> MWIVFDVDGVLIDVRESYD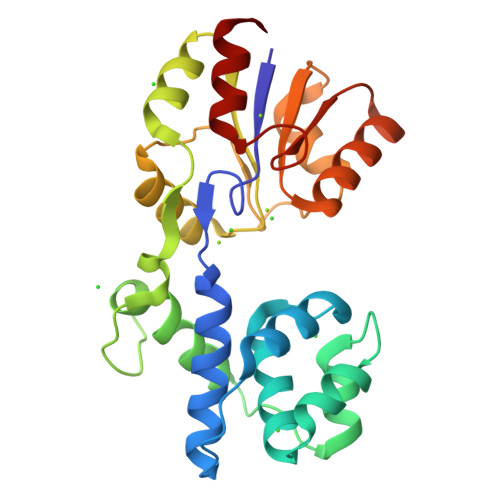EATKLTAEYFLGLFGVEREIKPEWVRELRRKGSFGDDFKVSEALILFALSGRAEELVEEFPEGGTIEWVREKFGFQVFGGSIERVFNTFYLGREYPERLFDFPGLWKKERPIVRRGLLERASKHFKLGVVTGRSALEMELAERIIGFKFENAVTREAYLKPDPRALWELVRGEPGVYIGDTINDELFVENYRGKYGDFDFVMVGRDVKDVNEFLENALEGG> MKSNDMNITVELTFFEPYRLVEWFDWDARKKSHSAMRGQAFAQWTWKGKGRTAGKSFITGTLVRSAVIKAVEELLSLNNGKWEGVPCCNGSFQTDESKGKKPSFLRKRHTLQWQANNKNICDKEEACPFCILLGRFDNAGKVHERNKDYDIHFSNFDLDHKQEKNDLRLVDIASGRILNRVDFDTGKAKDYFRTWEADYETYGTYTGRITLRNEHAKKLLLASLGFVDKLCGALCRIEVIKKSESPLPSDTKEQSYTKDDTVEVLSEDHNDELRKQAEVIVEAFKQNDKLEKIRILADAIRTLRLHGEGVIEKDELPDGKEERDKGHHLWDIKVQGTALRTKLKELWQSNKDIGWRKFTEMLGSNLYLIYKKETGGVSTRFRILGDTEYYSKAHDSEGSDLFIPVTPPEGIETKEWIIVGRLKAATPFYFGVQQPSDSIPGKEKKSEDSLVINEHTSFNILLDKENRYRIPRSALRGALRRDLRTAFGSGCNVSLGGQILCNCKVCIEMRRITLKDSVSDFSEPPEIRYRIAKNPGTATVEDGSLFDIEVGPEGLTFPFVLRYRGHKFPEQLSSVIRYWEENDGKNGMAWLGGLDSTGKGRFALKDIKIFEWDLNQKINEYIKERGMRGKEKELLEMGESSLPDGLIPYKFFEERECLFPYKENLKPQWSEVQYTIEVGSPLLTADTISALTEPGNRDAIAYKKRVYNDGNNAIEPEPRFAVKSETHRGIFRTAVGRRTGDLGKEDHEDCTCDMCIIFGNEHESSKIRFEDLELINGNEFEKLEKHIDHVAIDRFTGGALDKAKFDTYPLAGSPKKPLKLKGRFWIKKGFSGDHKLLITTALSDIRDGLYPLGSKGGVGYGWVAGISIDDNVPDDFKEMINKTEMPLPEEVEESNNGPINNDYVHPGHQSPKQDHKNKNIYYPHYFLDSGSKVYREKDIITHEEFTEELLSGKINCKLETLTPLIIPDTSDENGLKLQGNKPGHKNYKFFNINGELMIPGSELRGMLRTHFEALTKSCFAIFGEDSTLSWRMNADEKDYKIDSNSIRKMESQRNPKYRIPDELQKELRNSGNGLFNRLYTSERRFWSDVSNKFENSI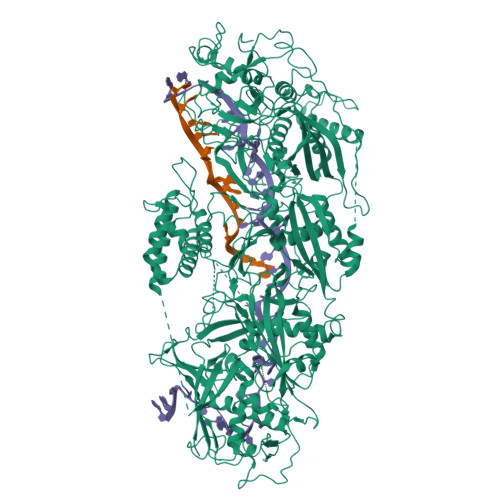DYKREILRCAGRPKNYKGGIIRQRKDSLMAEELKVHRLPLYDNFDIPDSAYKANDHCRKSATCSTSRGCRERFTCGIKVRDKNRVFLNAANNNRQYLNNIKKSNHDLYLQYLKGEKKIRFNSKVITGSERSPIDVIAELNERGRQTGFIKLSGLNNSNKSQGNTGTTFNSGWDRFELNILLDDLETRPSKSDYPRPRLLFTKDQYEYNITKRCERVFEIDKGNKTGYPVDDQIKKNYEDILDSYDGIKDQEVAERFDTFTRGSKLKVGDLVYFHIDGDNKIDSLIPVRISRKCASKTLGGKLDKALHPCTGLSDGLCPGCHLFGTTDYKGRVKFGFAKYENGPEWLITRGNNPERSLTLGVLESPRPAFSIPDDESEIPGRKFYLHHNGWRIIRQKQLEIRETVQPERNVTTEVMDKGNVFSFDVRFENLREWELGLLLQSLDPGKNIAHKLGKGKPYGFGSVKIKIDSLHTFKINSNNDKIKRVPQSDIREYINKGYQKLIEWSGNNSIQKGNVLPQWHVIPHIDKLYKLLWVPFLNDSKLEPDVRYPVLNEESKGYIEGSDYTYKKLGDKDNLPYKTRVKGLTTPWSPWNPFQVIAEHEEQEVNVTGSRPSVTDKIERDGKMV>MRVLALSAVFLVAS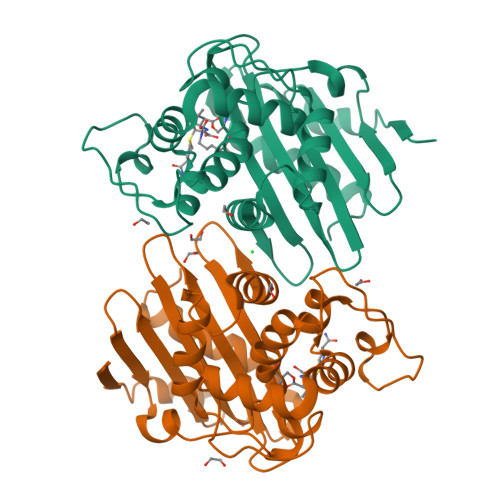IIGMPAVAKEWQENKSWNAHFTEHKSQGVVVLWNENKQQGFTNNLKRANQAFLPASTFKIPNSLIALDLGVVKDEHQVFKWDGQTRDIATWNRDHNLITAMKYSVVPVYQEFARQIGEARMSKMLHAFDYGNEDISGNVDSFWLDGGIRISATEQISFLRKLYHNKLHVSERSQRIVKQAMLTEANGDYIIRAKTGYSTRIEPKIGWWVGWVELDDNVWFFAMNMDMPTSDGLGLRQAITKEVLKQEKIIP[8x]> GMRCNERNKKKAIFSNDDFSGEDTLMEDHLQLREKLSEDIEMIKASLKNNLVCSTLNDNEILTLSNYMQFFVFKGGDLVIKQGEKGSYFFIINSGKFDVYVNDKKVKSMGKGSSFGEAALIHNTQRSATIMAETDGTLWGVQRSTFRATLKQLSNRNFNENRSFIDSVSVFDMLTEAQKNMITNACVIQMFKPGETIVKQGDYGDVLFILKEGKATVFINDKEIRVLNKGSYFGERALLYDEPRSATIIAKEPTACASICRKLLNIVLGNLQVVLFRNIMTEALQQSEIFRQFSAEQLNDLADTAIVRDYPANYHILHKDKVKSVKYLIVLEGKVELFLDDESIGILTRGKSFGDQYVLNQKQKFRHTVKSLDVCKIALITESCLADCLGDNNIDASIDHNNKKSIIKKMYIFRYLSEQQCNLLIEAFRTTRYEEGDYIIQEGEVGSRFYIIKNGEVEVTKNGKRLRTLGKNDYFGERALLYDEPRTASIISKATSVECWFVDKSVFLQIIQGPMLTHLEERIKMQDTKVEMHELETERIIGRGTFGTVKLVHHKPTQIRYALKCVSKRSIISLNQQNNIKLEREITAENDHPFIIRLVRTFKDSNCFYFLTELVTGGELYDAIRKLGLLSKPQAQFYLGSIILAIEYLHERNIVYRDLKPENILLDKQGYVKLIDFGCAKKIQGRAYTLVGTPHYMAPEVILGKGYGCTVDIWALGVCLYEFICGPLPFGNDQEDQLEIFRDILTGQLTFPDYVSDQDSINLMKRLLCRLPQGRIGCSINGFKDIKEHAFFGNFNWDKLAGRLLEPPLVSKGETYAEDIDIKQIEEEDALNEGEPLDGDDSWDVDF

Previous work has demonstrated that one particular kinase, known as cyclic guanosine-3′,5′-monophosphate (cGMP)-dependent protein kinase, or protein kinase G (PKG), has essential roles in multiple stages of the parasite life cycle. Selective pharmacological inhibition of Plasmodium falciparum PKG (PfPKG) blocks the egress of merozoites and gametes from erythrocytes, as well as inhibits the motility of ookinetes in the mosquito and invasion of hepatocytes by sporozoites. The cellular functions of parasite PKG are regulated by allosteric and cooperative binding of cGMP, similarly to how mammalian PKG is activated. In contrast, PKG enzymes of Plasmodium and other apicomplexan parasites have an extended N-terminal domain that features four CNBs upstream of the KD and are monomeric, resulting in an effective regulatory stoichiometry of 4:1.

We report herein the structure of cGMP-free PKG from Plasmodium parasites, the causative agents of malaria, one of the world’s deadliest infectious diseases. Here, we describe the complete atomic structure of PKG from two human malaria parasite species, P. falciparum and Plasmodium vivax. The two orthologs are 92% identical in sequence; furthermore, alignment of their structures resulted in rmsds of 0.8 Å—representing negligible differences. In the Plasmodium PKG crystal structures, each protomer in the dimers can be described as four CNBs, which, together with the N lobe of the KD, form a pentagonal arrangement, with the KD C lobe locked in the center. Interestingly, all three Plasmodium structures display a swapped domain arrangement, in which the N terminus of each protomer in the dimer interacts with the active site of the other. All three of our Plasmodium PKG structures feature an activation loop that is both in its open conformation and unphosphorylated—an uncommon combination previously observed in rho kinases and rho-associated kinases such as ROCK and MRCK. Although the domain-swapped dimer in our crystal structures suggests the intriguing possibility of an intermolecular regulatory system (in which each protomer extends N-terminal residues to block the substrate-binding site of its dimeric partner), the totality of our biochemical and biophysical data indicates cGMP-free (i.e., inactive) Plasmodium PKG to be predominantly a monomer.>CSTVSPGVLAGIVVGDLVLTVLIALAVYFLGRL[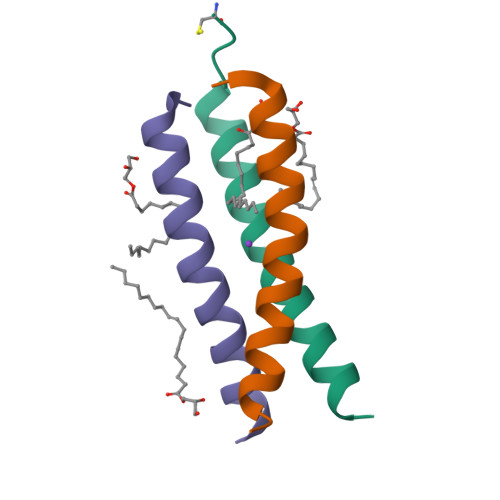3x]>[6x]HLPLIAITRNPVFPRFIKIIEVKNKKLVELLRRKVRLAQPYVGVFLKRDDSNESDVVESLDEIYHTGTFAQIHEMQDLGDKLRMIVMGHRRVHISRQLEVEPEEPEAENKHKPRRKSKRGKKEAEDELSARHPAELAMEPTPELPAEVLMVEVENVVHEDFQVTEEVKALT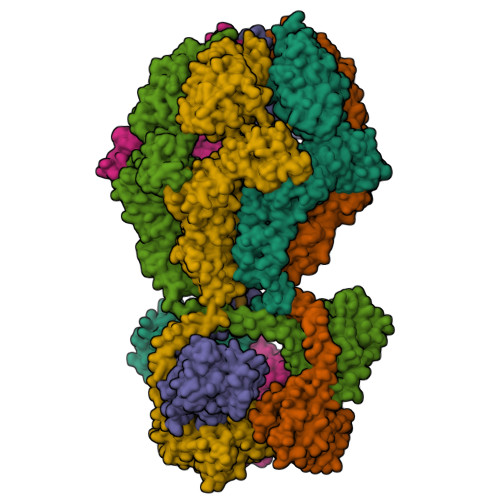AEIVKTIRDIIALNPLYRESVLQMMQAGQRVVDNPIYLSDMGAALTGAESHELQDVLEETNIPKRLYKALSLLKKEFELSKLQQRLGREVEEKIKQTHRKYLLQEQLKIIKKELGLEKDDKDAIEEKFRERLKELVVPKHVMDVVDEELSKLGLLDNHSSEFNVTRNYLDWLTSIPWGKYSNENLDLARAQAVLEEDHYGMEDVKKRILEFIAVSQLRGSTQGKILCFYGPPGVGKTSIARSIARALNREYFRFSVGGMTDVAEIKGHRRTYVGAMPGKIIQCLKKTKTENPLILIDEVDKIGRGYQGDPSSALLELLDPEQNANFLDHYLDVPVDLSKVLFICTANVTDTIPEPLRDRMEMINVSGYVAQEKLAIAERYLVPQARALCGLDESKAKLSSDVLTLLIKQYCRESGVRNLQKQVEKVLRKSAYKIVSGEAESVEVTPENLQDFVGKPVFTVERMYDVTPPGVVMGLAWTAMGGSTLFVETSLRRPQDKDAKGDKDGSLEVTGQLGEVMKESARIAYTFARAFLMQHAPANDYLVTSHIHLHVPEGATPKDGPSAGCTIVTALLSLAMGRPVRQNLAMTGEVSLTGKILPVGGIKEKTIAAKRAGVTCIVLPAENKKDFYDLAAFITEGLEVHFVEHYREIFDIAFP>[2x]MLNTTFANAKFANPFMNASGVHCMTIEDLEELKASQAGAYITKSSTLEKREGNPLPRYVDLELGSIASMGLPNLGFDYYLDYVLKNQKENAQE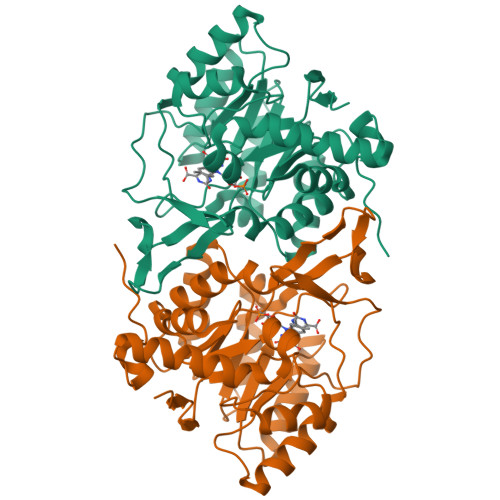GPIFFSIAGMSAAENIAMLKKIQESDFSGITELNLSCPNVPGKPQLAYDFEATEKLLKEVFTFFTKPLGVKLPPYFDLVHFDIMAEILNQFPLTYVNSVNSIGNGLFIDPEAESVVIKPKDGFGGIGGAYIKPTALANVRAFYTRLKPEIQIIGTGGIETGQDAFEHLLCGATMLQIGTALHKEGPAIFDRIIKELEEIMNQKGYQSIADFHGKLKSL> GSHMSYQKVPNSHKEFTKFCYEVYNEIKISDKEFKEKRAALDTLRLCLKRISPDAELVAFGSLESGLALKNSDMDLCVLMDSRVQSDTIAL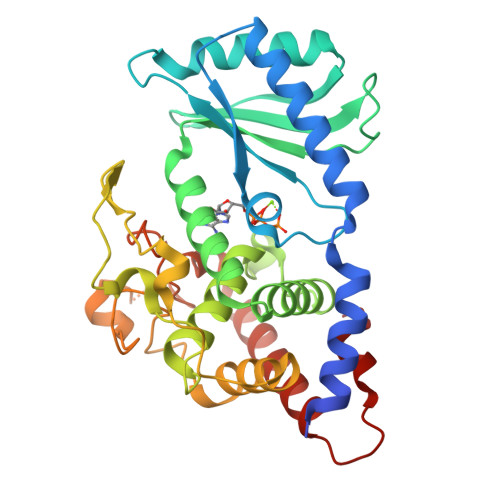QFYEELIAEGFEGKFLQRARIPIIKLTSDTKNGFGASFQCDIGFNNRLAIHNTLLLSSYTKLDARLKPMVLLVKHWAKRKQINSPYFGTLSSYGYVLMVLYYLIHVIKPPVFPNLLLSPLKQEKIVDGFDVGFDDKLEDIPPSQNYSSLGSLLHGFFRFYAYKFEPREKVVTFRRPDGYLTKQEKGWTSATEHTGSADQIIKDRYILAIEDPFEISNNVGRTVSSSGLYRIRGEFMAASRLLNSRSYPIPYDSLFEEA> GGCGUGGUCCGUUCAACUCGUUCCUCGAAAGAGGA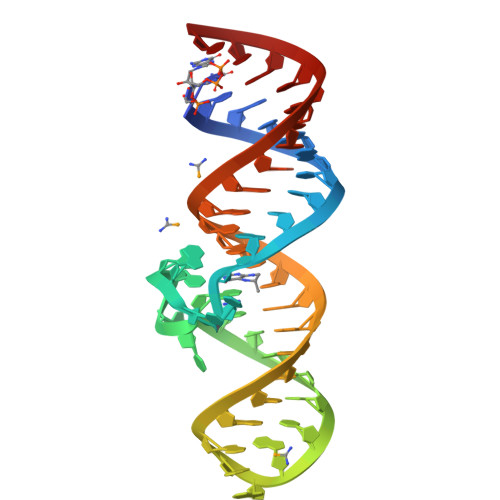ACUACGGGAGACGCC> MGSDKIHHHHHHMKNSFFSKFTPKEPKFFPLLKQLSDVLSASSVLLVESMEHDLPTERADYYKQIKDMEREGDRLTHLIFDELSTTFITPFDREDIHDLASCMDDVIDGINSSAKRIVIYNPRPISESGKELSRLIHEEAINIGKAMDELETFRKNPKPLRDYCTQLHDIENQADDVYE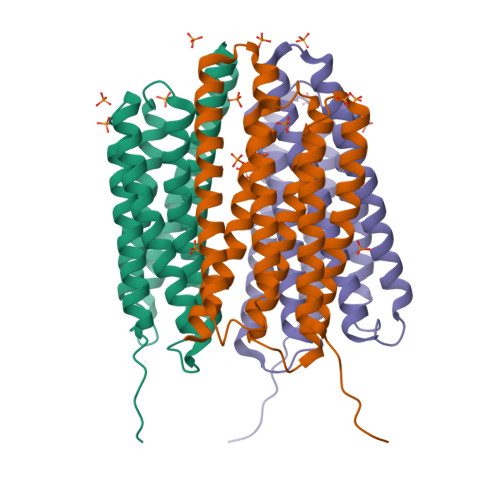LFITKLFEEEKDCIELIKIKEIMHELEKTTDAAEHVGKILKNLIVKYS> MKTQVAIIGAGPSGLLLGQLLHKAGIDN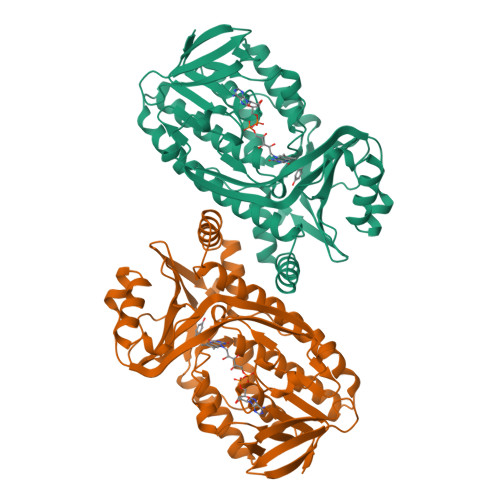VILERQTPDYVLGRIRAGVLEQGMVDLLREAGVDRRMARDGLVHEGVEIAFAGQRRRIDLKRLSGGKTVTVYGQTEVTRDLMEAREASGATTVYQAAEVRLHDLQGERPYVTFERDGERLRLDCDYIAGCDGFRGISRQSIPAERLKVFERVYPFGWLGLLADTPPVSHELIYANHPRGFALCSQRSATRSRYYVQVPLTEKVEDWSDERFWTELKARLPAEVAEKLVTGPSLEKSIAPLRSFVVEPMQHGRLFLAGDAAHIVPPTGAKGLNLAASDVSTLYRLLLKAYREGRGELLERYSAICLRRIWKAERFSWWMTSVLHRFPDTDAFSQRIQQTELEYYLGSEAGLATIAENYVGLPYEEIE> MTYVQDGNKSELRKAKRQLVTVIDLNKCLGCQTCTVACKNIWTKRPGTEHMRWNNVTTYPGKGYPRDYERKGGGFLRGEPQPGVLPTLIDSGDDFQFNHKEVFYEGKGQTVHFHPTSKSTGKDPAWGYNWDEDQGGGKWPNPFFFYLARMCNHCTNPACLAACPTGAIYKREDNGIVLVDQERCKGHRHCVEACPYKAIYFNPVSQTSEKCILCYPRIEKGIANACNRQCPGRVRAFGYLDDTTSHVHKLVKKWKVALPLHAEYGTGPNIYYVPPMGARGFGEDGEITDKTRIPLDVLEGLFGPEVKRVLAVLHTERENMRAGRGSELMDLLISKKWSDRFGGFTNDPL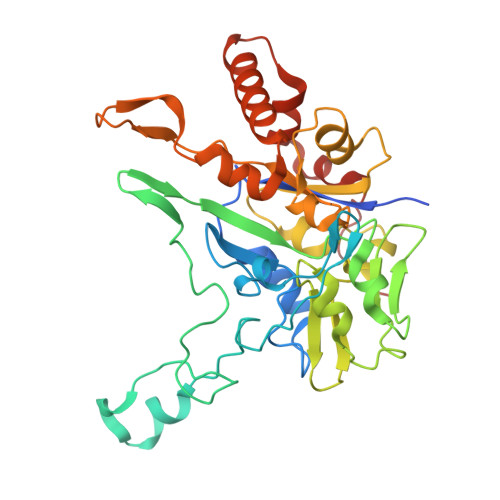TQS>[8x]GSSHHHHHHMKSLVGVIMGSTSDWET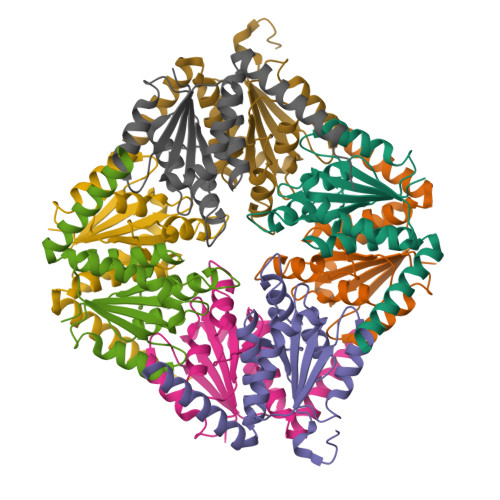MKYACDILDELNIPYEKKVVSAHRTPDYMFEYAETARERGLKVIIAGAGGAAHLPGMVAAKTNLPVIGVPVQSKALNGLDSLLSIVQMPGGVPVATVAIGKAGSTNAGLLAAQILGSFHDDIHDALELRREAIEKDVREGSELV> AMSRSRPELGDWSSPAELAELQRSQLPRVLAQALRSPFYAARYRGTTPPRTADDFAGVEVTAKQDLRDQYPFGMLAVGREHLATYHESSGTAGEPTASYYTEEDWTDLAERFARKWTGIHPSDTFLVRTPYGLVITGHLAQAAGRLRGATVVPGDARSLATPLSRMVRVLKTLDVTLTWCNPTEITMLAAAAKAAGLRPDQDFPHLRAMFTAAEPLTEVRRRRLSEIWGGIPVVEEYGSTETGTIAGQCPEGRMHLWADRAIFEVYDPRTGTLSEAGRGQMVVTPLYRDAMPLLRYNLADDVEVSTDPCGCGWLLPTVTVLGRAGTGHRIGPATVTQQRLEELVFSLPAAYEVMFWRAKAHPDVLELEFEAPEPVRQRAVKELGAALDRELGVPHRITGLAPGTLVPAEALTAQRD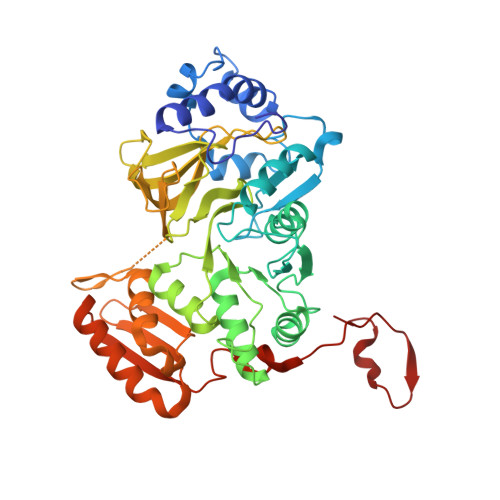ILKARYLFAEDEDWDKAVMYF> MRIILLGAPGAGKGTQAQFIME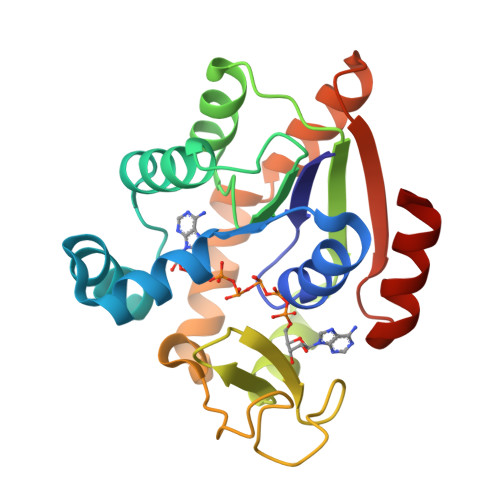KYGIPQISTGDMLRAAIKSGSELGKQAKDIMDAGKLVTDEIIIALVKERICQEDSRNGFLLDGFPRTIPQADAMKEAGINVDYVLEFDVPDELIVDRIVGRRVHAPSGRVYHVKFNPPKVEGKDDVTGEELTTRKDDQEETVRKRLVEYHQMTAPLIGYYSKEAEAGNTKYAKVDGTKPVCEVRADLEKILG>MHHHHHHMQVQDLTGAALDYWVATAEGHEVPRADASG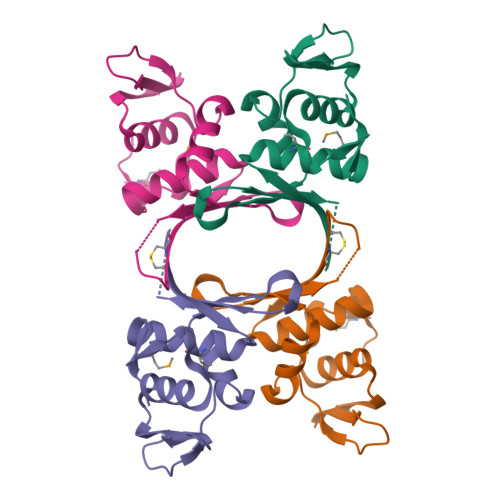CTSIREPGGVPTPFAPSSSWADGGPIVERLPFAGFERDGGRGAWRAVLHRAVPAAGERCTFNQSGPTLLIAAMRTLVASTFGDDVPDL[2x]The methylation of the ε-amino group of lysine residues is catalyzed by protein lysine methyltransferases (PKMTs), which can introduce up to three methyl groups with high specificity using S-Adenosyl-L-methionine (AdoMet) as methyl group donor. The SET-domain containing protein 2 (SETD2, also called KMT3A) PKMT was first identified as huntingtin interacting protein 1 (HYPB, HIP-1). It has a size of 230 kDa corresponding to 2564 amino acids and can add up to three methyl groups to K36 of histone H39. The ability for trimethylation of H3K36 makes SETD2 unique, because no other trimethyltransferase for this lysine residue is known in human cells. The structures of SETD2 in complex with H3K36 variant peptides and S-Adenosyl-L-homocysteine (AdoHcy) revealed that the substrate peptide is positioned in a deep binding channel in the catalytic SET domain where several contacts between the enzyme and the substrate peptide are formed.

To understand the molecular basis of the super-substrate methylation by SETD2, we determined the crystal structure of the human SETD2 catalytic domain (aa 1435–1711) bound to AdoHcy and the super-substrate peptide containing a target lysine to methionine mutation (ssK36M). We observed clear electron density for the ssK36M peptide and a cofactor product corresponding to AdoHcy, feasibly formed from AdoMet under the crystallization conditions. The ssK36M peptide is in an extended conformation, and AdoHcy is surrounded by residues of the SET and post-SET domains. The super-substrate carries four amino acid exchanges (A31R, T32F, K37R, and H39N) with respect to the canonical H3K36 peptide. Although not completely resolved by electron density, the side chain of ssK36M R31 (in its most likely conformation ttt18033,34) may form a salt bridge with the side chain of Glu1674. The aromatic F32 side chain of ssK36M is inserted into a shallow pocket formed by the side chains of Glu1674 and Gln1676 making more extensive hydrophobic interactions than T32 of H3K36M. In conclusion, the substituted residues in the super-substrate ssK36M interact with SETD2 mainly through the post-SET domain loop and the α6 helix of the SETD2 catalytic domain. Slotting of the F32 phenyl ring into a pocket between the Glu1674 and Gln1676 and possible interactions involving the guanidine moieties of R31 and R37 provide a plausible rationale for the enhanced methylation activity by SETD2 due to a tighter binding affinity between the super-substrate peptide and SETD2.

> MHHHHHHSSGRENLYFQGETSVPPGSALVGPSCVMDDFRDPQRWKECAKQGKMPCYFDLIEENVYLTERKKNKSHRDIKRMQCECTPLSKDERAQGEIACGEDCLNRLLMIECSSRCPNGDYCSNRRFQRKQHADVEVILTEKKGWGLRAAKDLPSNTFVLEYCGEVLDHKEFKARVKEYARNKNIHYYFMALKNDEIIDATQKGNCSRFMNHSCEPNCETQKWTVNGQLRVGFFTTKLVPSGSELTFDYQFQRYGKEAQKCFCGSANCRGYLGGENRVSIRAAGGKMKKERSRK;> APRFGGVMRPNRYR> STDASYNADIKEERDAAEGPMAHGIPALNAGALDEARAYATVDSANTDEEVSVAVDVTNLAVVAYRAGSNSYFHAAAPGSSLSHLFSRSSQHTLGFDNTYGDMAQAAGSNRKAIPLGAAALESGIASLNSKNPLARTLMVIIQMLVEAARFRYIQNNVDVSIETQSAFAADAAMISLENNWANLSALVQGSSGGQGTFASSATLQNAEDEPIIVDAVYHPTVAAVLALM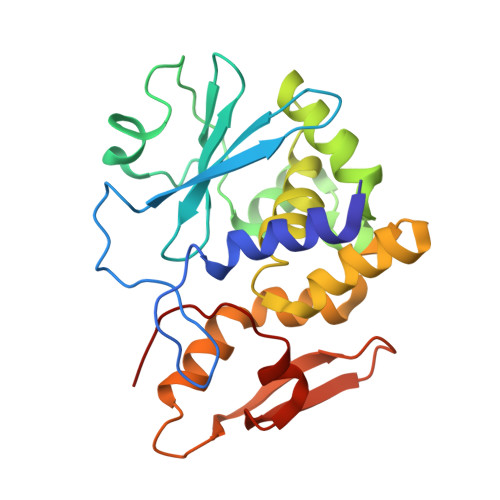LRKAC> R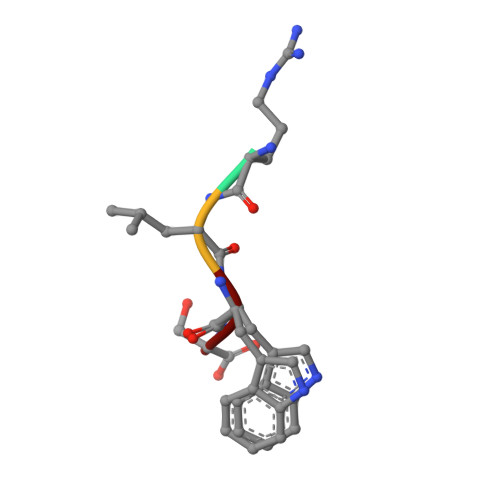LWS The only de novo biosynthetic pathway to generate dTTP (2′-deoxythymidine-5′-triphosphate) requires reductive methylation of dUMP (2′-deoxyuridine-5′-monophosphate) to dTMP (2′-deoxythymidine-5′-monophosphate) by TS. The TS enzyme is an obligatory homodimer whose subunits associate with nanomolar affinity to form a dimer that adopts an asymmetric conformation upon substrate binding. Inhibition of TS leads to the cessation of DNA replication and thymineless death of proliferating cells, which renders the enzyme an attractive target for cancer chemotherapy. Ligand-free TS protein binds its own mRNA and thereby represses translation.

To gain direct insight into the molecular recognition of mRNA by hTS, we attempted co-crystallization of the enzyme with oligonucleotide constructs representing the TS site 1 motif. X-ray data sets were collected and structures determined for crystals grown at low salt (100 mM buffer) as well as high salt (1.75 M ammonium sulphate) concentration. Molecular replacement with previously published hTS coordinates furnished structures with the enzyme adopting either of the previously observed active and inactive conformations of the loop regions about I108-G129 and A181-A197; however, each without RNA bound. In the active conformation, the catalytic C195 is located in the active site, while it resides at the dimer interface in the inactive conformation. Previously, it had been proposed that hTS functions as a metabolic enzyme in the active conformation but as a nucleic acid-binding protein in the inactive state. Structure comparison of native and substrate-liganded hTS suggested that nucleic acid-binding might be achieved in the inactive but not the active conformation of the enzyme. In the inactive conformation, the K107–E128 peptide is disordered and allows ligand access to the G84–K104 helix–loop–helix motif. Although the crystallography effort furnished structures of the protein in both the active and inactive conformation, co-crystallization of an hTS–RNA complex remained elusive.

> MPVAGSELPRRPLPPAAQERDAEPRPPHGELQYLGQIQHILRCGVRKDDRTGTGTLSVFGMQARYSLRDEFPLLTTKRVFWKGVLEELLWFIKGSTNAKELSSKGVKIWDANGSRDFLDSLGFSTREEGDLGPVYGFQWRHFGAEYRDMESDYSGQGVDQLQRVIDTIKTNPDDRRIIMCAWNPRDLPLMALPPCHALCQFYVVNSELSCQLYQRSGDMGLGVPFNIASYALLTYMIAHITGLKPGDFIHTLGDAHIYLNHIEPLKIQLQREPRPFPKLRILRKVEKIDDFKAEDFQIEGYNPHPTIKMEMAVHHHHH Cellobiohydrolases (CBHs) play key roles in degradation of crystalline cellulose, which is the homopolymer of β-1,4-linked glucose and fundamental component of plant cell wall. High hydrolytic activity of CBHs against crystalline cellulose is achieved by the unique structure of the catalytic domain (CD), which consists of tunnel-shaped substrate-binding sites covered by loops. The unique function of CBH is a unidirectional movement on cellulose surface coupled with processive hydrolysis of the cellulose chain into cellobiose, the minimum repeating unit. In contrast, GH6 CBH from the bacterium C. fimi (CfCel6B) has CBM2-CBD and three fibronectin type 3 domains (FN3s) as a linker between CD and CBD.

We solved a crystal structure of CfCel6B CD with 1.3 Å resolution, to clarify the structural difference between CfCel6B and TrCel6A CDs. In the determined crystal structure of CfCel6B CD, we confirmed that the Val43, which is close to the N terminus of CfCel6B (without signal peptide) and mutated to Cys in the single-molecule fluorescence imaging, was located in the opposite side of the catalytic site. Overall structure of CfCel6B CD was similar to that of the TrCel6A CD except for the additional subsite and loops. In the crystal structure, CfCel6B has additional substrate-binding site (subsite) constructed by Trp303 at plus side, the same as TfCel6B. This additional subsite is stabilized by two loops (shown in blue) which are not found in TrCel6A. Near the product-binding site, a pair of exit loops has been also found in CfCel6B and TfCel6B. The exit loop 1 (shown in green) was capping the end of the substrate-binding tunnel. This exit loop 1 of CfCel6B is 4 amino acids shorter than that of TfCel6B, indicating that the tunnel of CfCel6B is more open than that of TfCel6B. In addition, the exit loop 2 (shown in cyan) of CfCel6B showed more open conformations compared with that of TfCel6B. The Ser105 and the N-terminal loop of CfCel6B, crystallized without ligand, stayed outside of the cleft. The slow component for CD, which was not found in TrCel6A, has been observed in CfCel6B. This result strongly suggests that CfCel6B CD has higher processivity than TrCel6A CD by the additional subsite and loops observed in the crystal structure.

> MAPVHVDNPYAGAVQYVNPTWAASVNAAAGRQSADPALAAKMRTVAGQPTAVWMDRISAITGNADGNGLKFHLDNAVAQQKAAGVPLVFNLVIYDLPGRDCFALASNGELPATDAGLARYKSEYIDPIADLLDNPEYESIRIAATIEPDSLPNLTTNISEPACQQAAPYYRQGVKYALDKLHAIPNVYNYIDIGHSGWLGWDSNAGPSATLFAEVAKSTTAGFASIDGFVSDVANTTPLEEPLLSDSSLTINNTPIRSSKFYEWNFDFDEIDYTAHMHRLLVAAGFPSSIGMLVDTSRNGWGGPNRPTSITASTDVNAYVDANRVDRRVHRGAWCNPLGAGIGRFPEATPSGYAASHLDAFVWIKPPGESDGASTDIPNDQGKRFDRMCDPTFVSPKLNNQLTGATPNAPLAGQWFEEQFVTLVKNAYPVIGGTTPVEDLVAPTIEGRFGGHHHHHH>[2x]MVRSFIYEAFQIPSGSMMPTLLIGDFILVEKFAYG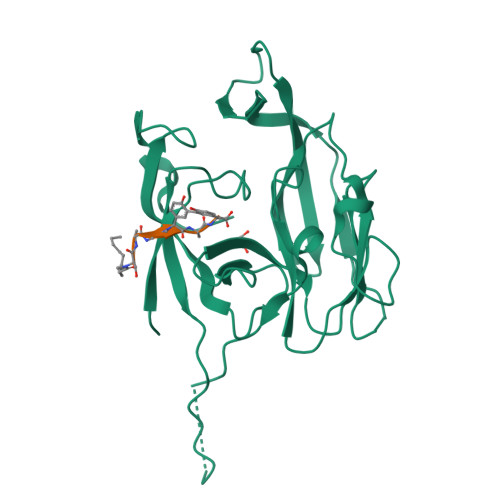IKDPIYQKTLIETGHPKRGDIVVFKYPEDPKLDYIKRAVGLPGDKVTYDPVSKELTIQPGCSSGQACENALPVTYSNVEPSDFVQTFSRRNGGEATSGFFEVPKNETKENGIRLSERKETLGDVTHRILTVPIAQDQVGMYYQQPGQQLATWIVPPGQYFMMGDNRDNSADSRYWGFVPEANLVGRATAIWMSFDKQEGEWPTGLRLSRIGGIH;>[2x]SAGGAY> MNPDNYLYLSALLFTIGAAGVLLR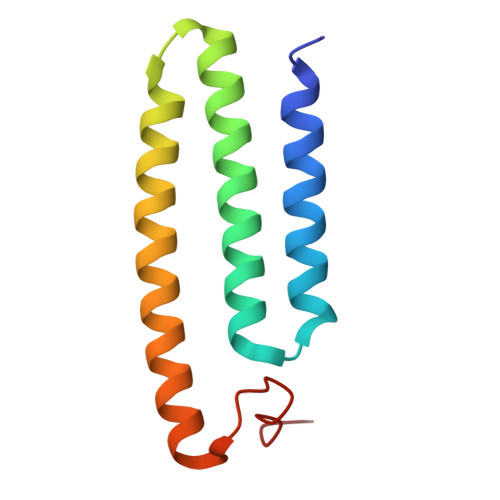RNAIVMFMCVELMLNAANLAFVNFSRMHGQLDGQVVAFFTMVVAACEVVVGLAIIMAIFRTRRSASVDDANLLKH>MNHKVHMAEEGAVAVCVRVRPLNSREESLGETAQVYWKTDNNVIYQVDGSKSFNFDRVFHGNETTKNVYEEIAAPIIDSAIQGYNGTIFAYGQTASGKTYTMMGSEDHLGVIPRAIHDIFQKIKKFPDREFLLRVSYMEIYNETITDLLCGTQKMKPLIIREDVNRNVYVADLTEEVVYTSEMALKWITKGEKSRHYGETKMNQRSSRSHTIFRMILESREKGEPSNCEGSVKVSHLNLVDLAGSERAAQTGAAGVRLKEGCNINRSLFILGQVIKKLSDGQVGGFINYRDSKLTRILQNSLGGNPKTRIICTITPVSFDETLTALQFASTAKYMKNTPYVNEVSGSHHHHH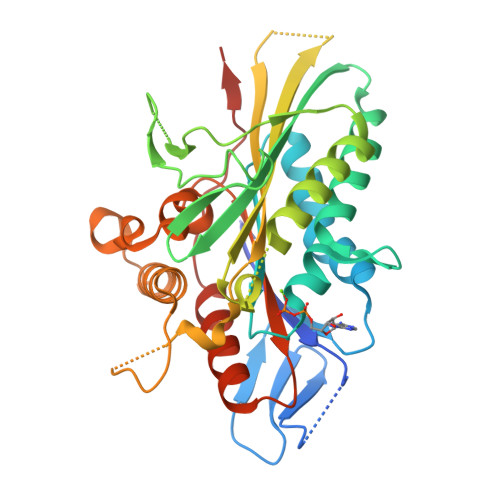H[2x]> AAAAAAAAAAAAAAAAAAAAAA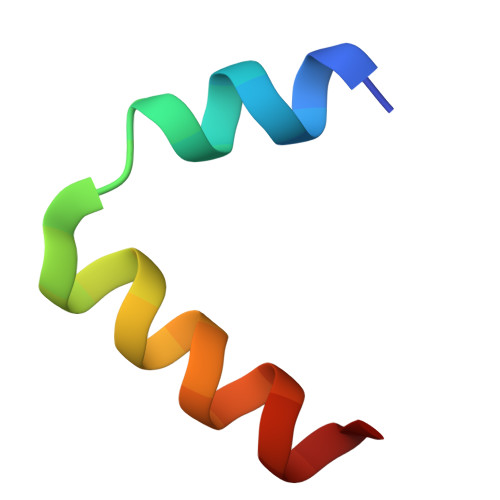AAAAA PYRUVAMIDE 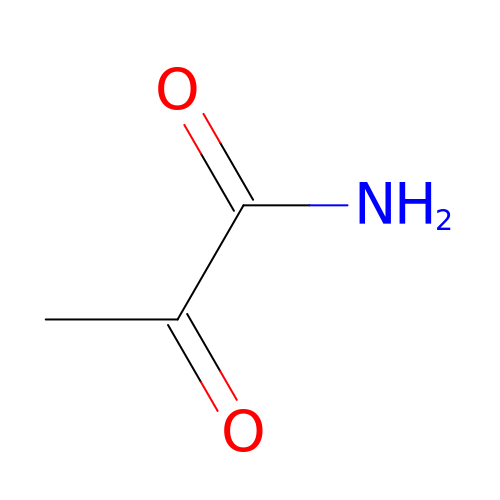| C3 H5 N O2 | FPOLWERNILTNDK-UHFFFAOYSA-N>[2x]LGSENDVIELDDVANIMFYGEGEVGDNHQKFMLIFDTGSANLWVPSKKCNSSGCSIKNLYDSSKSKSYEKDGTKVDITYGSGTVKGFFSKDLVTLGHLSMPYKFIEVIDTDDLEPIYSSVEFDGILGLGWKDLSIGSIDPIVVELKNQNKIDNALFTFYLPVHDVHAGYL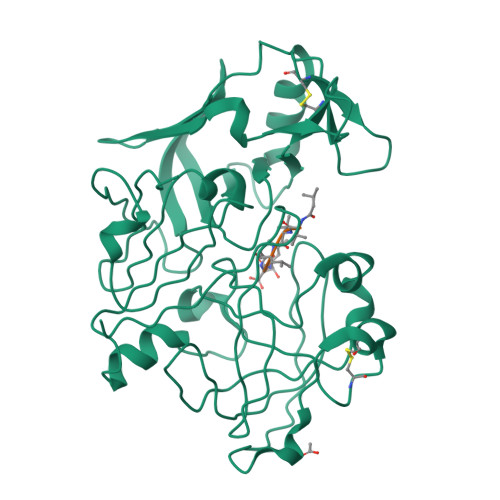TIGGIEEKFYEGNITYEKLNHDLYWQIDLDVHFGKQTMEKANVIVDSGTTTITAPSEFLNKFFANLNVIKVPFLPFYVTTCDNKEMPTLEFKSANNTYTLEPEYYMNPILEVDDTLCMITMLPVDIDSNTFILGDPFMRKYFTVFDYDKESVGFAIAKN> QSQQTFXNLWRL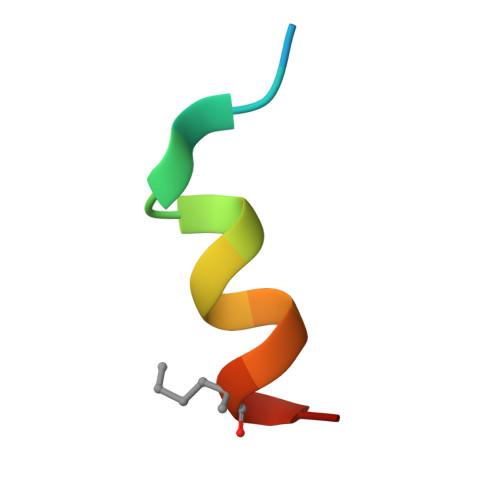ELQNX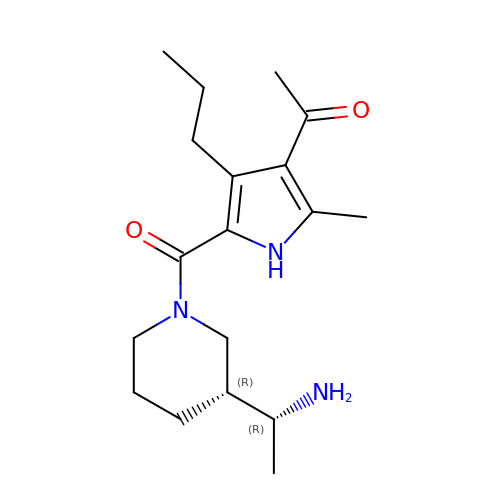1-[5-[(3~{R})-3-[(1~{R})-1-azanylethyl]piperidin-1-yl]carbonyl-2-methyl-4-propyl-1~{H}-pyrrol-3-yl]ethanone | C18 H29 N3 O2 | OWYUHPPXERUPEI-BXUZGUMPSA-N>STGLWWEEVEDSYEREDVQKKTFTKWVNAQFSKFGKQHIENLFSDLQDGRRLLDLLEGLTGQKLPKEKGSTRVHALNNVNKALRVLQNNNVDLVNIGSTDIVDGNHKLTLGLIWNIILHWQVKNVMKNIMAGLQQTNSEKILLSWVRQSTRNYPQVNVINFTTSWSDGLALNALIHSHRPDLFDWNSVVSQQSATQRLEHAFNIA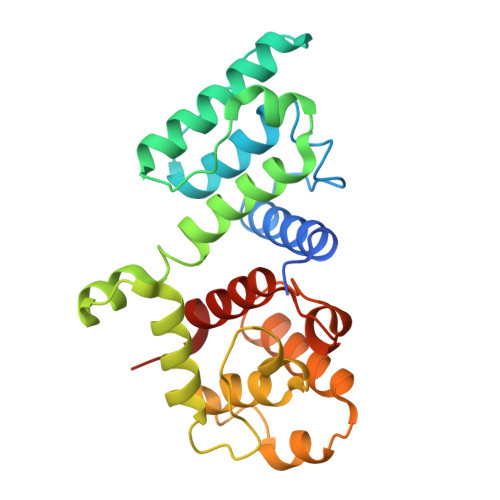RYQLGIEKLLDPEDVDTTYPDKKSILMYITSLFQVLPQQVSIE[4x]> MSTTTRPFVLPGETIDPSLVPTHPKHPLRLGPGLRHVPPSDIIPTVAGQLITNLNKNSMWVEYNSQRYVPTQNDLVLAQVLRSTQDSYLCLITPHTPPATLPHLAFESATKKT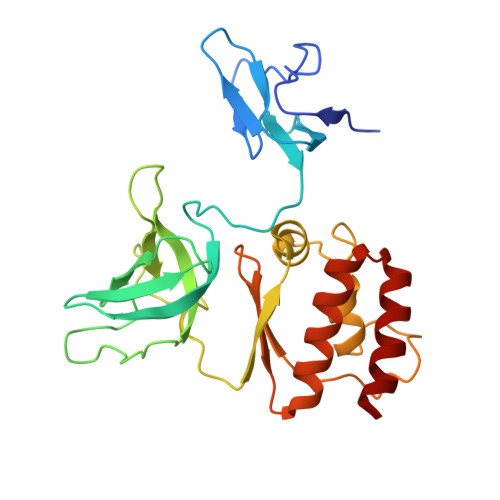RPQLQPGQLVYARVSLANRHMDPELECVNPSTGKADGLGPITGPGCVFEVSLGFARRLLMAKSREEGKVGVLEMLAGEDPSIGEAGAGLAFETAVGRNGRVWVGSEDVKTVIIVGRALQETDRGNLTIEGQRKLVRRLLREMR>[12x]GSHMGPSGAADKAGTRENQPAVVHLQGQGSAIQVKNDLSGGVLNDWS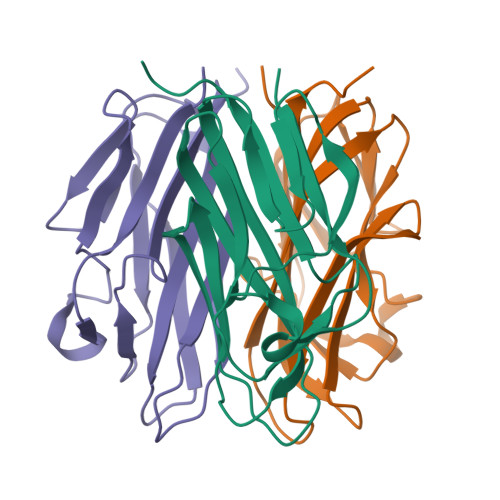RITMNPKVFKLHPRSGELEVLVDGTYFIYSQVEVYYINFTDFASYEVVVDEKPFLQCTRSIETGKTNYNTCYTAGVCLLKARQKIAVKMVHADISINMSKHTTFFGAIRLGEAPAS> GPGSMQRASRLKRELHMLATEPPPGITCWQDKDQMDDLRAQILGGANTPYEKGVFKLRVIIPERYPFE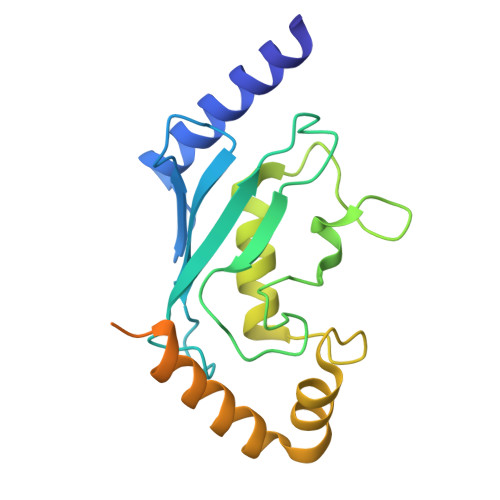PPQIRFLTPIYHPNIDSAGRICLDVLKLPPKGAWRPSLNIATVLTSIQLLMSEPNPDDPLMADISSEFKYNKPAFLKNARQWTEKHARQKQKADEEEMLDNLPEAGDSRVHNSTQKRKASQLVGIEKKFHPDV The periplasmic chaperone SilF has been identified as part of an Ag(I) detoxification system in Gram-negative bacteria. Biophysical and biochemical analysis of proteins comprising the sil gene cluster has been limited to date, with sequence homology used to infer function and the proposed resistance mechanism, after comparison with the more extensively studied cus and cue systems. Such analysis is consistent with the model that the SilF is a periplasmic metal-binding chaperone capable of binding both Ag(I) and Cu(I) ions and shuttling them to the SilCBA complex to aid metal ion detoxification. The protein has a β-barrel topology composed of five β-stands arranged in the β1-β2-β3-β5-β4-β1, similar to that observed for Cu(I) chaperone CusF. The X-ray crystal structures show that the metal ion–binding site is formed from strictly conserved residues His63, Trp71, Met74, and Met76 located at one end of the β-barrel.

Cocrystallization of SilF38-120 with either Ag(I) or Cu(I) under anaerobic conditions yields an orthorhombic unit cell with three protein chains per asymmetric unit and each chain with one metal ion bound close to one end of the β-barrel. In both the Ag(I)- and Cu(I)-bound structures, the metal ion is coordinated with distorted tetrahedral geometry through the donor groups NE2 of His63 and the two thiol groups of Met74 and Met76. The Cu(I) coordination geometry within the binding site is noticeably different than that of Ag(I) where the fourth coordination position of the Cu(I) ion is occupied by a water molecule. The Trp71 is now blocked from directly interacting with the metal. Furthermore, the side-chain of Met74 adopts a different rotameric conformer compared to the apo and Ag(I) structures. Such flexibility allows the protein to provide ligands at shorter coordination distances so as to accommodate the smaller ion. By contrast, the conformations of Met76 and His63 remain unchanged between structures. Ag(I) has a dissociation constant (Kd) of 7.6 nM, whereas Cu(I) binds with a Kd of 30 nM: both determined free energies values were within experimental error of each other meaning that the affinity of SilF38-120 for either metal ion are very similar in size. The differing role of water in the two binding mechanisms allows an adaptability of the binding site to accommodate the two different cations with similar affinity.

>[2x]MVQQVIRGSGVVKAIDMNSKKITISHEAIPAVGWPAMTMRFTFVNADDAIDAINALKTGNHVDFSFIQQGNISLLKSIN;>MVQQVIRGSGVVKAIDMNSKKITISHEAIPAVGWPAMTMRFTFVNADDAIDAINALKTGNHVDFSFIQQGNISLLKSINV[4x]> MTFPGDTAVLVLAAGPGTRMRSDTPKVLHTLAGRSMLSHVLHAIAKLAPQRLIVVLGHDHQRIAPLVGELADTLGRTIDVALQDRPLGTGHAVLCGLSALPDDYAGNVVVTSGDTPLLDADTLADLIATHRAVSAAVTVLTTTLDDPFGYGRILRTQDHEVMAIVEQTDATPSQREIREVNAGVYAFDIAALRSALSRLSSNNAQQELYLTDVIAILRSDGQTVHASHVDDSALVAGVNNRVQLAELASELNRRVVAAHQLAGVTVVDPATTWIDVDVTIGRDTVIHPGTQLLGRTQIGGRCVVGPDTTLTDVAVGDGASVVRTHGSSSSIGDGAAVGPFTYLRPGTALGADGKLGAFVEVKNST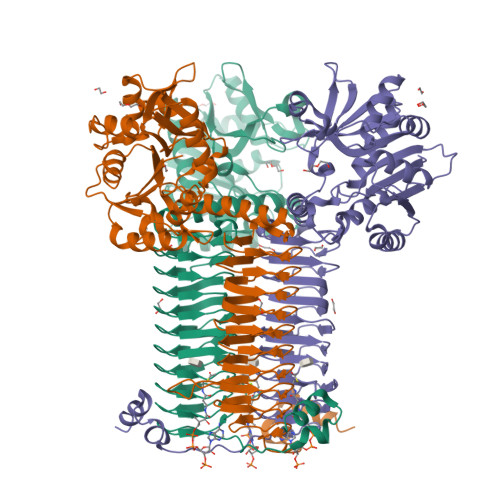IGTGTKVPHLTYVGDADIGEYSNIGASSVFVNYDGTSKRRTTVGSHVRTGSDTMFVAPVTIGDGAYTGAGTVVREDVPPGALAVSAGPQRNIENWVQRKRPGSPAAQASKRASEMACQQPTQPPDADQTP>[2x]RKPKTGILMLNMGGPETLGDVHDFLLRLFLDRDLMTLPIQNKLAPFIAKRLTPKIQEQYRRIGGGSPIKIWTSKQGEGMVK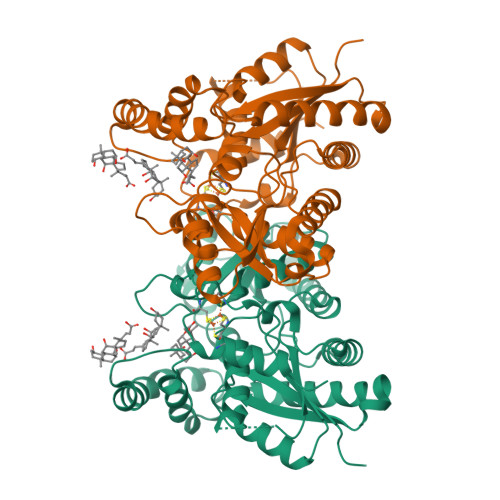LLDELSPNTAPHKYYIGFRYVHPLTEEAIEEMERDGLERAIAFTQYPQYSCSTTGSSLNAIYRYYNQVGRKPTMKWSTIDRWPTHHLLIQCFADHILKELDHFPLEKRSEVVILFSAHSLPMSVVNRGDPYPQEVSATVQKVMERLEYCNPYRLVWQSKVGPMPWLGPQTDESIKGLCERGRKNILLVPIAATSDHIETLYELDIEYSQVLAKECGVENIRRAESLNGNPLFSKALADLVHSHIQSNELCSKQLTLSCPLCVNPVCRETKSFFTSQQL> ANAIAVGSERSADGKGMLLANPHFPWNGA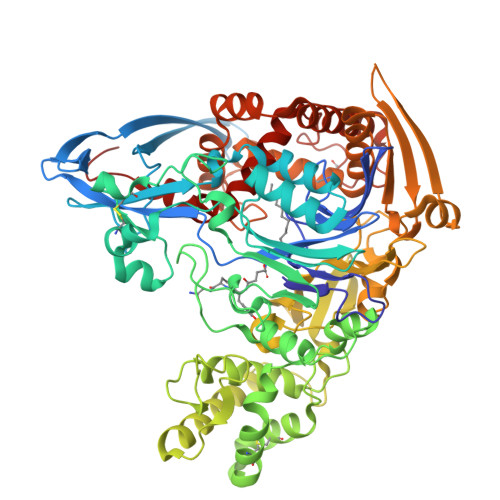MRFYQMHLTIPGRLDVMGASLPGLPVVNIGFSRHLAWTHTVDTSSHFTLYRLALDPKDPRRYLVDGRSLPLEEKSVAIEVRGADGKLSRVEHKVYQSIYGPLVVWPGKLDWNRSEAYALRDANLENTRVLQQWYSINQASDVADLRRRVEALQGIPWVNTLAADEQGNALYMNQSVVPYLKPELIPACAIPQLVAEGLPALQGQDSRCAWSRDPAAAQAGITPAAQLPVLLRRDFVQNSDDSAWLTNPASPLQGFSPLVSQEKPIGPRARYALSRLQGKQPLEAKTLEEMVTANHVFSADQVLPDLLRLCRDNQGEKSLARACAALAQWDRGANLDSGSGFVYFQRFMQRFAELDGAWKEPFDAQRPLDTPQGIALDRPQVATQVRQALADAAAEVEKSGIPDGARWGDLQVSTRGQERIAIPGGDGHFGVYNAIQSVRKGDHLEVVGGTSYIQLVTFPEEGPKARGLLAFSQSSDPRSPHYRDQTELFSRQQWQTLPFSDRQIDADPQLQRLSIREGGLAADIRWTAYGVPHIRAKDERGLGYGIGYAYARDNACLLAEEIVTARGERARYFGSEGKSSAELDNLPSDIFYAWLNQPEALQAFWQAQTPAVRQLLEGYAAGFNRFLREADGKTTSCLGQPWLRAIATDDLLRLTRRLLVEGGVGQFADALVAAAPPGAE> MGSHHHHHHGSLEVLFQGPHMASNSLNSKLEPTLENLENLDVSAFQAPEDLLDGCRIYLCGFSGRKLDKLRRLINSGGGVRFNQLNEDVTHVIVGDYDDELKQFWNKSAHRPHVVGAKWLLECFSKGYMLSEEPYIHANYQPVEIPVSHQPESKAALLKKKNSSFSKKDFAPSEKHEQADEDLLSQYENGSSTVVEAKTSEARPFND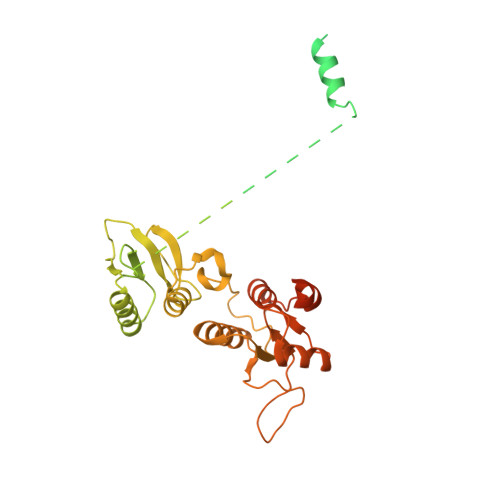STHAEPLNDSTHISLQEENQSSVSHCVPDVSTITEEGLFSQKSFLVLGFSNENESNIANIIKENAGKIMSLLSRTVADYAVVPLLGCEVEATVGEVVTNTWLVTCIDYQTLFDPKSNPLFTPVPVMTGMTPLEDCVISFSQCAGAEKESLTFLANLLGASVQEYFVRKSNAKKGMFASTHLILKERGGSKYEAAKKWNLPAVTIAWLLETARTGKRADESHFLIENSTKEERSLETEITNGINLNSDTAEHPRRAWSHPQFEK7-cyano-7-deazainosine | C12 H12 N4 O5 | 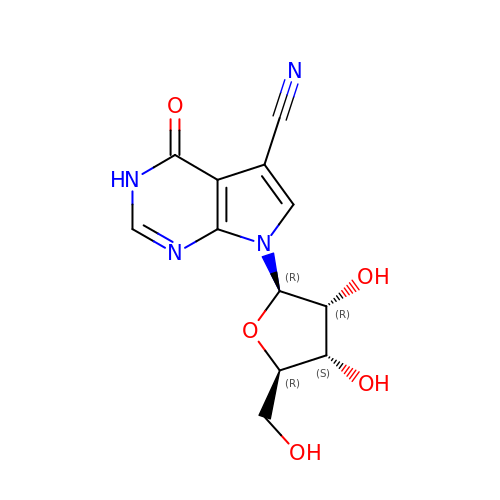SKDKFLFSBDYEDO-WOUKDFQISA-N>MAVPETRPNHTIYINNLNEKIKKDELKKSLHAIFSRFGQILDILVSRSLKMRGQAWVIFKEVSSATNALRSMQGFPFYDKPMRIQYA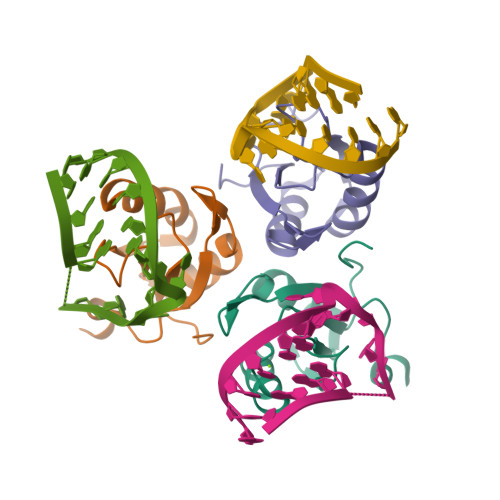KTDSDIIAKMK[3x]Myxovirus resistance (Mx) proteins are key mediators of interferon-induced innate immune response in vertebrates. MxA restricts a broad range of RNA viruses, including the influenza virus, whereas MxB was recently shown to inhibit human immune deficiency viruses.

To verify their architectures, we determined a 2.9 Å nucleotide-free crystal structure of a monomeric MxA construct (termed MxAMO1) containing the following modifications: (i) deletion of N-terminal 32 residues and part of L4S (residues 533–561 inclusive), (ii) point mutations in interface 1 (I376S, K614S, L617S and L620S) and interface 2 (M527D). The overall folding and domain distribution of MxAMO1 shows a high consistency with MxAFL. Moreover, the infrastructure of MxAMO1 hinge 1 remains intact, and a higher quality of diffraction data compared to that of MxAFL revealed that the previously unexplained K644 of α3B, a conserved residue among Mx proteins, is involved in the BSE-hinge 1 association by forming a salt bridge with D363 of L1BS. Altogether, the MxAMO1 structure indicates that disruption of the oligomerization interfaces of the stalk does not affect the architecture of MxA. To explain this result, we reviewed the crystal structure of MxAMO1 at the corresponding region. Hinge 1 is substantially attached to the proximal end of the stalk via a hydrophobic network which allows very limited relative movement. On the other side, salt bridge pairs involving D363-R640 and E632-K644 from BSE and hinge 1 may act as a key bracket that supports the BSE from hinge 1 while allowing a certain level of elasticity. Thus, mutation of the central R640 would engender the collapse of this bracket, hence the structural defects of MxA. Sites 352 and 500 span 35.3 and 35.6 Å in crystal structures of apo MxAMO2 and MxAFL, respectively.

>PGSVAENNLCSQYEEKVRPCIDLIDSLRALGVEQDLALPAIAVIGDQSSGKSSVLEALSGVALPRGSGIVTRCPLVLKLKKLVNEDKWRGKVSYQDYEIEISDASEVEKEINKAQNAIAGEGMGISHELITLEISSRDVPDLTLIDLPGITRVAVGNQPADIGYKIKTLIKKYIQRQETISLVVVPSNVDIATTEALSMAQEVDPEGDRTIGILTKPDLVDKGTEDKVVDVVRNLVFHLKKGYMIVKCRGQQEIQDQLSLSEALQREKIFFENHPYFRDLLEEGKATVPCLAEKLTSELITHICKSLPLLENQIKETHQRITEELQKYGVDIPEDENEKMFFLSDKINAFNQDITALMQGEETVGEEDIRLFTRLRHEFHKWSTIIENNFQEGHKILSRKIQKFENQAAAAELPGFVNYRTFETIVKQQIKALEEPAVDMLHTVTDMVRLAFTDVSIKNFEEFFNLHRTAKSKIEDIRAEQEREGEKLIRLHFQDEQIVYGAFQSSSATDSSMEEIFQHLMAYHQEASKRISSHIPLIIQFFMLQTYGQQLQSAMSQLSQDKDTYSWLLKERSDTSDKRKFLKERLARLTQARRRLAQFPG[2x]>MKKIEAIVRAEKFPEVKAALEERGFYGMTVTDVKGRGQQGGMQIQFRGRTMEVTLLPKVKLEI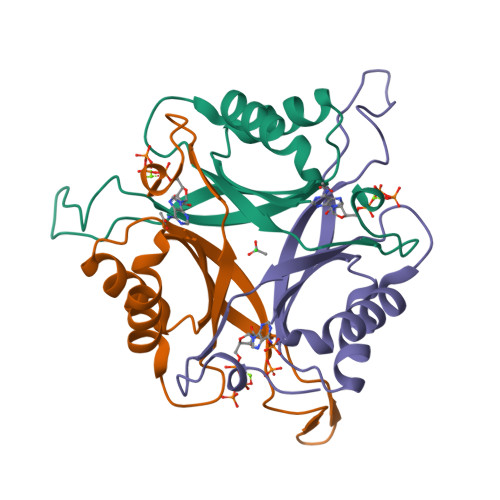VVKDDAVEEVIGLIVNSAFTGSPGDGKIFIIPVEDVVRIRTGERGDDSLEHHHHHH[3x]> MLSQNVAKTTVPSYYMIRTNLPQRKPQNQWEGVYYFGGITKRQRHLILLQRKREREARMRAFSASCSNLLRLLEGDTQEQQQAKTQTIQLSSPHGPFDLAIRLAQHGLYQQASRIVDELHQQRALRMSHYGLLIDALSAPCLGQRILYGSAQCDPALTYKLLGDENGEERAQEAHRWFDMAFALLTTECRMSGSEHRLPQATAAATHLVNALMRALLTCGYTHVSAVPDAVYDRMGLMGISPTISTYELVMLALSLQGNMKEAESVFSFLRRHHNEHVTIGSFNALLLGHRECRQFDRCDAIWQELVDRRWPRASTLTAELYLRSIVDHSYTPTSGPLQRFGNINVVEKKKIPLVLAQMDDLGIPRAHLSRPLMDEVEDALRKFHIYKSRYYEWGRAVKQFNFIEFRRRNGWMYDLHLMKNTTKQVGPLRDFNQPDATQAPVATVEIPAFFNERPAWEQPPLEETLYVTESRERYDDVRSGDIYEDRTRSLHDRSPTWMNEVPETRYDHLYGVNH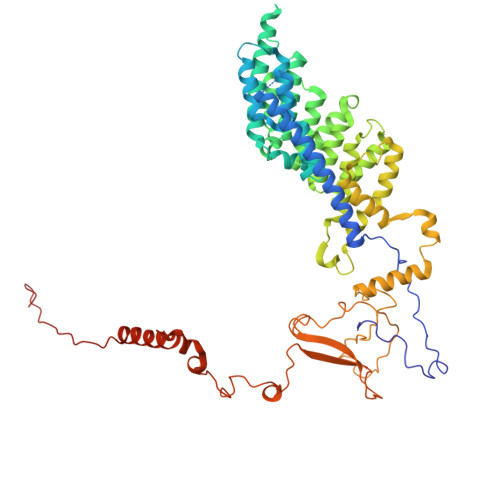PDIAKIGIRRHLNAEYVNRKEVVERDAALMKKNLSTGRRLRRKVESSRTHRNAGSMSGAAPASASR> VTAKELAEKAGAAAGLKAGDIHGMKIVIEGLKALKVDTLKSGIFNSFVQNSHYTEVTGLAIAIDTEMNEVCSATYIGIHPICVVREKLGVIPKAGGTMVKQKDAITNVLKQALEKATQSAEALSETTAED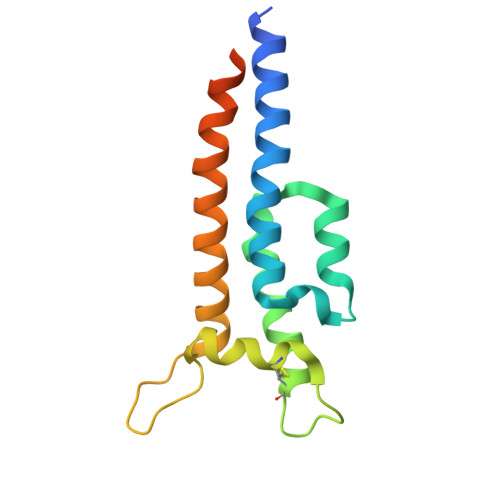VAAKLTAQKTGAINT N-[3-(4-CHLOROPHENYL)-1-{N'-CYANO-N-[3-(DIFLUOROMETHOXY)PHENYL]CARBAMIMIDOYL}-4,5-DIHYDRO-1H- PYRAZOL-4-YL]-N-ETHYL-2-HYDROXYACETAMIDE | C22 H21 Cl F2 N6 O3 | 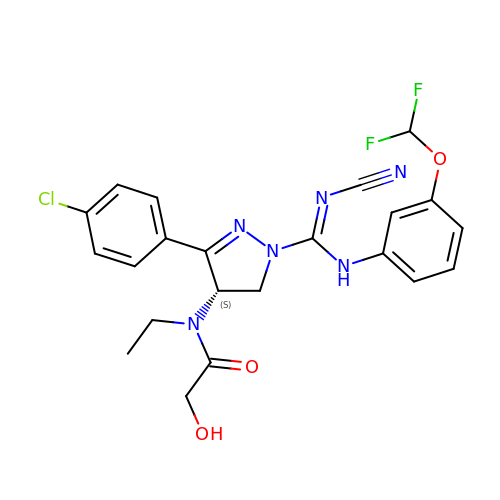GZPIECMFJJLDAB-SFHVURJKSA-N> GLGDELEEVIVEKTKQTVASISSGPKHTQKVPILTANETGATMPVLPSDSIETRTTYMHFNGSETDVECFLGRAACVHVTEIQNKDATGIDNHREAKLFNDWKINLSSLVQLRKKLELFTYVRFDSEYTILATASQPDSANYSSNLVVQAMYVPPGAPNPKEWDDYTWQSASNPSVFFKVGDTSRFSVPYVGLASAYNCFYDGYSHDDAETQYGITVLNHMGSMAFRIVNEHDEHKTLVKIRVYHRAKHVEAWIPRAPRALPYTSIGRTNYPKNTEPVIKKRKGDIKSY;> SPNVEACGYSDRVQQITLGNSTITTQEAANAVVC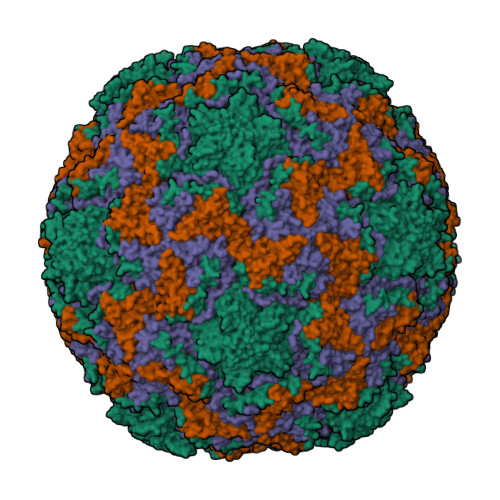YAEWPEYLPDVDASDVNKTSKPDTSVCRFYTLDSKTWTTGSKGWCWKLPDALKDMGVFGQNMFFHSLGRSGYTVHVQCNATKFHSGCLLVVVIPEHQLASHEGGNVSVKYTFTHPGERGIDLSSANEVGGPVKDVVYNMNGTLLGNLLIFPHQFINLRTNNTATIVIPYINSVPIDSMTRHNNVSLMVIPIAPLTVPTGATPSLPITVTIAPMCTEFSGIRSKSIVPQ;> GLPTTTLPGSGQFLTTDDRQSPSALPNYEPTPRIHIPGKVHNLLEIIQVDTLIPMNNTHTKDEVNSYLIPLNANRQNEQVFGTNLFIGDGVFKTTLLGEIVQYYTHWSGSLRFSLMYTGPALSSAKLILAYTPPGARGPQDRREAMLGTHVVWDIGLQSTIVMTIPWTSGVQFRYTDPDTYTSAGFLSCWYQTSLILPPETTGQVYLLSFISACPDFKLRLMKDTQTISQTVALTE;> GAQVSTQKSGSHENQNILTNGSNQTFTVINYYKDAASTSSAGQSLSMDPSKFTEPVKDLMLKGAPALN>MTTTSPLHFVTLLGSLRKASFNAAVARALPEIAPEGIAITPLGSIGTFPHYSQDVQEEGFPAPVLTMAQQIATADAVVIVTPEYNYSVPGVLKNAIDWLSRVSPQPLAGKPVALVTASPGMIGGARAQYHLRQSLVFLDAYVLNRPEAMIGQVTGKVDAQTLELSDVATREFLARQLDALAALARTLSPRAITHH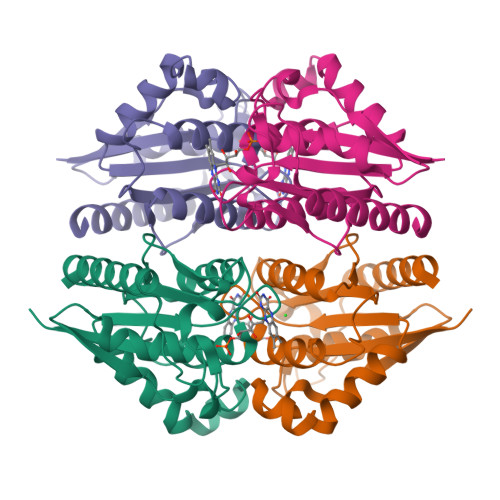HHHH[4x]> DPFAGDPPRHPGLRVNSQKPFNAEPPAELLAERFLTPNELFFTQNHLPVP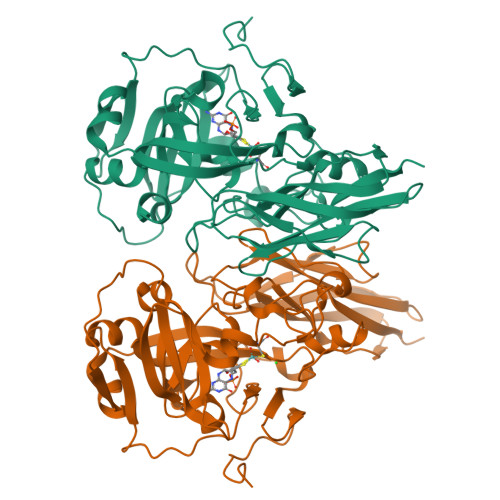AVEPSSYRLRVDGPGGGTLSLSLAELRSRFPKHEVTATLQCAGNRRSEMSRVRPVKGLPWDIGAISTARWGGARLRDVLLHAGFPEELQGEWHVCFEGLDADPGGAPYGASIPYGRALSPAADVLLAYEMNGTELPRDHGFPVRVVVPGVVGARSVKWLRRVAVSPDESPSHWQQNDYKGFSPCVDWDTVDYRTAPAIQELPVQSAVTQPRPGAAVPPGELTVKGYAWSGGGREVVRVDVSLDGGRTWKVARLMGDKAPPGRAWAWALWELTVPVEAGTELEIVCKAVDSSYNVQPDSVAPIWNLRGVLSTAWHRVRVSVQD>[2x]MLSVENKVVAPPMVYIAGEEMTRYACDLVVKSWLEPYFDLSQWEYFDLSCVNRDNTNDQVLRDAVTAGQRIGAIFKEPTITPSAIQKKAFGLKNSLGSPNGAMRAGWNGITISRDTIHIDGIELGYKRPVFFERHAVGGEYGAGWSKVGRGTLLTTYLPSDGRDPFVVDKRDLTDQHNVVVTYHNPYDNVEPLAHLFFQRCLDANITPYVVTKKTVFKWQEGFWAVMKDVFDEHYKSRFEEKGLLQACGGDLQHLISDAATMQLIRWTDGGFGMAAHNYDGDMLTDQIAQVHRSPGFITSNLVGKAPDGSLIKEFEASHGTVSDLWNDHLAGKETSLNPLGLVEAIVGALQHAAVLDAEKNPDDEHKVKARDQIFNFTTTLRTAMHNTFRYGQGTRDMSGPSGYTTEDFVRKVAWRLQRYLDAQYDEAPPPQLGEPSRKLRRNYDIDEEAINGLFQKYDKNGDGFIDFEEFTRMLVKMNLAPLLTKKEKEKKPDV

Isocitrate dehydrogenase (IDH) plays a critical role in the tricarboxylic acid (TCA) cycle and catalyzes the oxidative decarboxylation of isocitrate to generate CO2 and α-ketoglutarate (α-KG) with divalent metal ions (Mg2+ or Mn2+) while reducing NAD(P)+ to NAD(P)H. In accordance with the preference of coenzyme, IDHs are divided into two forms: NAD+-dependent IDH (EC 1.1.1.41, NAD-IDH) and NADP+-dependent IDH (EC 1.1.1.42, NADP-IDH). In the present study, we investigated the overexpression, purification, and detailed biochemical characteristics of a type II homodimeric NAD-IDH from P. tricornutum (PtIDH1). To our knowledge, PtIDH1 is the first eukaryotic homodimeric NAD-IDH structure proposed in the type II subfamily, and it exhibits a unique EF-hand domain at the C-terminal. Enzymatic characterization has revealed that recombinant PtIDH1 is a completely NAD+-dependent IDH and exhibits allosteric regulation by isocitrate, similar to eukaryotic mitochondrial NAD-IDHs from O. tauri, S. cerevisiae, Pisum sativum, and Solanum tuberosum.

The apo form crystal structure of PtIDH1 was determined at 2.8 Å resolution in space group P212121, and the asymmetric unit contained two monomers that form a dimer. Each subunit of PtIDH1 in the final refined structure missed several amino acid residues, including Met1-Val4 and Lys487-Val495 (15 residues). The monomer of PtIDH1 mainly consists of three distinct domains: a large domain, a small domain, and a clasp domain. In addition, a unique EF-hand domain is observed at the C-terminal domain of Gln424-Lys486, which is composed of a helix‒loop‒helix conformation. As with all structured homodimeric IDHs, there are two clefts on each side of the structure, which are formed by the large and small domains of one subunit and the small domain of the adjacent domain. The putative active sites are located in these two cleft regions. Additionally, PtIDH1 contained two insertions (Ala84-Gly91 and Ser323-Ala331) in the large domain, specifically forming two α-helices (α4 and α11) at the active site. Moreover, the dimeric interface area of PtIDH1 (4082 Å2) was larger than that of HcIDH (3638 Å2), and at least a 1700 Å2 interface area was provided by the EF-hand domain of PtIDH1 at the C-terminal. Therefore, the dimerization was formed through the unique C-terminal EF-hand domain in PtIDH1. The structure reveals that PtIDH1 EF-hand loop contains several residues (Asp459, Asn461, Asp463, Phe465, Asp467, and Glu470) that are aligned well with Ca2+-coordinating residues conserved in other EF-hand loops, indicating that PtIDH1 EF-hand loop binds to Ca2+ by canonical coordinating mechanism.> MIAPLILYLDVPFTTFRESHAREMGKTYPVPPPATVYGMLLSLVGETNVYRHCGVELAIAMLSSPKKSRILRQMRRFKNADFSHPENVIPCYQEILSNLKCLIWVRSDEEKIQPSLRERIQLAFDHPELVRRFGCLFLGESDQLIKTIKLAREDYLEGVRQWAIRDNRGRLTLPYWVDHVGSRNTRFLRYRIEEMDRLSPPDLAWTMVQSPI;> MTAILIQSEEYVDLTFKLRGAPIPLDNGYLTYAALSRICPPLHELKSIGIHPIAGIPTRNNLLELTAQSRLKIRIYHQQIPLIYPYLAGQAFHIGQNFYQLDIPDYKPLISSESVYSRLVIIKGFQDSTNFIEAVQRQMDNLGIQGKIELLTRQDGTPQRRQLTINKEGKQFKVRGFGVKISELNPEDSLTLQEQGIGGKRKMMCGIFVPATRSKEEEET;>[6x]MMTQKKNDSNIPNYYLYGTVLTRYGLASLNHDIRRGNKTILQKGYWNNGKIHSFVGSSAIRWALRFYLQKQGYLVNRVWDEEEHINRLTSEDFDPEKFYDDDIFGFALLESAETEEDTSTTKRKKKQTKTSTPNQRMGALGMNMAVSLTPYDGAVKLGAKSGREKDSTSLHFTEYHATRYQYYFGIDATHLKDFSRILPMIDGIMNLPKVGGSSNIFNYPFCPDSLVFQWTNHFASYISYCFEYCDPKSKEAKLSQEFIDEVECGQIDPSKLWIGGTIVKDLQQLDNFESSPLNKAHIYRNRNE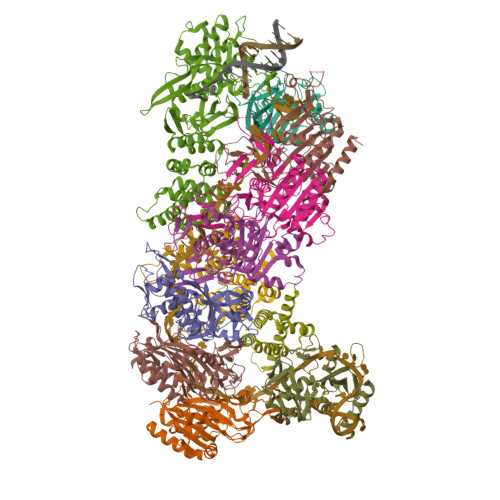MIEALKTVIKRDLGLEESK;> MHHHHHHHHIVSTQPKISLSLHAADTTIMHRVGMTGLYMTLKRLEKQYPLSRQRGGHISWFLTADTIELFWEGSDFIALSWLINESFQLDDTGLIHLVGLDNDRIDLRQKIHIHEGICGVFLRLNKFYQAGEIINTELRFEEKQVEYQYKSLTWYAHQTFAEKLCEADTQQLRHDYIQITSWLYLGGIVRHARTQNTTKLEEKPEYALALLFVPVVCHYCLLHIPSEDLKERKPHRYLVVIPEIKDFEDASQRRWRLQQLETKQFHVSSLGEAGLLYYSLDDIQPEVAYYQACQVWLYEKTNKASRQRTLMSIEEIKIDKNILITYQQVQKYFKTNYQIIKYKQIFIKVNPIRSLIADNLVKGIHWWSNFWEKLVIEDSKEYLFNQLFSNREGFIIMAENSEEDKQYLIFIKVFQQAMKGNFAKIYAKTEEGKDPPIKKKVERLRAELNYCYDELSFKEYLSDFLVRGGLNKYFNEHQEEIALLIKKSPWQEIRIWSLLAIASYKPKDKLTNRDDSSLSNNQKLEEVNDDSEEE;>MAENSEEDKQYLIFIKVFQQAMKGNFAKIYAKTEEGKDPPIKKKVERLRAELNYCYDELSFKEYLSDFLVRGGLNKYFNEHQEEIALLIKKSPWQEIRIWSLLAIASYKPKDKLTNRDDSSLSNNQKLEEVNDDSEEE[3x]> LTPLAQMAEGMERQD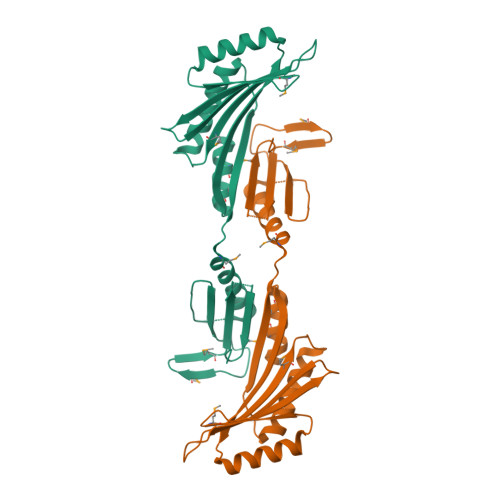VSIDKWTLHAKQNLSLTEKEFYQKVQRLKQEYRQYDWVIAREDKMIKAIGTYTDKKNRTSFRLQLVTTLKKHNPTSYLLYEQMSLETPDSWNDTYEQFERETLGIFQEKVVIFTCLNGHLDDNMNIVLQKKANQLLNEFQARSVEHVVEPNFVSISAFTDEWEEYIMTSKHKMNLQIALRSAGMGGKHTVTVGTPIVTTEY N-ALPHA-(2-NAPHTHYLSULFONYL)-N(3-AMIDINO-L-PHENYLALANINYL)ISOPIPECOLINIC 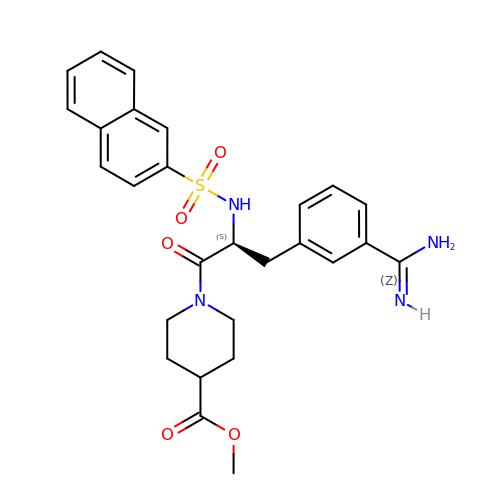ACID METHYL ESTER | C27 H30 N4 O5 S | JJLGQWCKMHPBEB-DEOSSOPVSA-N> SEACEMCRLGLPHGSFFELLRDW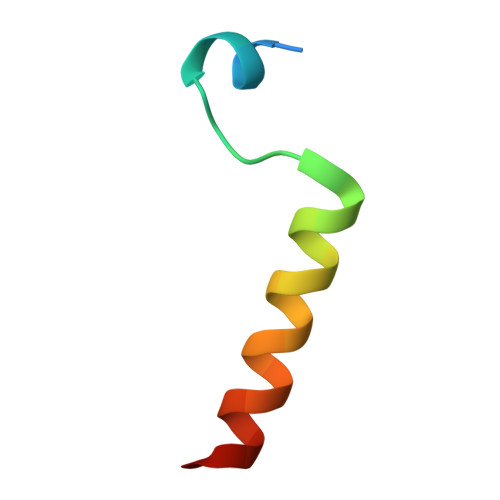KKIEEFRNKS> MKTLVHVASVEKGRSYEDFQKVYNAIALKLREDDEYDNY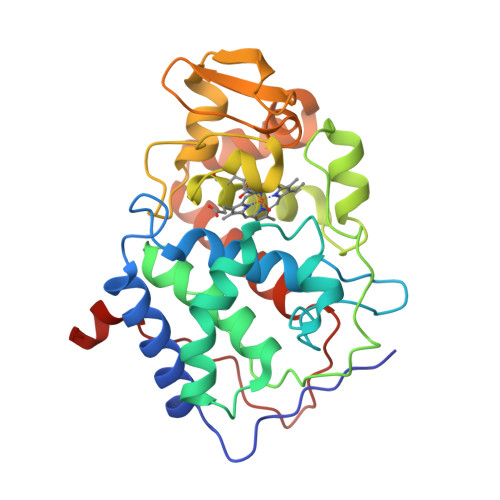IGYGPVLVRLAWHISGTWDKHDNTGGSYGGTYRFKKEFNDPSNAGLQNGFKFLEPIHKEFPWISSGDLFSLGGVTAVQEMQGPKIPWRCGRVDTPEDTTPDNGRLPDADKDAGYVRTFFQRLNMNDREVVALMGAHALGKTHLKNSGYEGPWGAANNVFTNEGYLNLLNEDWKLEKNDANNEQWDSKSGYMMLPTDYSLIQDPKYLSIVKEYANDQDKFFKDFSKAFEKLLENGITFPKDAPSPFIFKTLEEQGL> MELIKGQALFLELDKKDFLSLKNNDKNIPTFA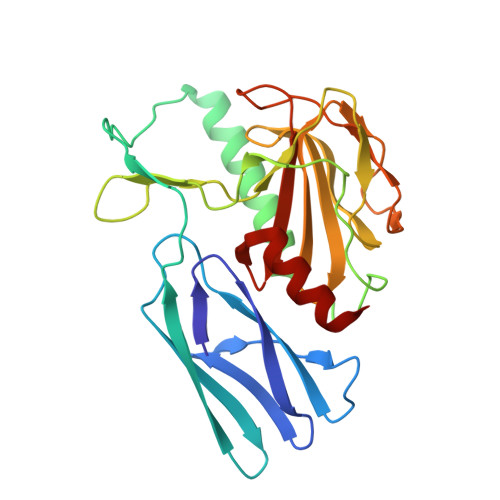HPKNQEKILAIFSLPYKNPPQNTKLIAFYKDKKEEIFIKTLEGNYKSEKLQVENKKIFPPKTIQERIAKELKEANAIYSSYTPKALFNGAFNIPLNSFITSDFGKARTFNEKVASYHSGTDFRAATGTPIYAANSGVVKIAKDRYFAGNSVVIDHGFGIYSQYYHLSKIDVKVGQKIKKGELIGLSGASGRVSGPALHFGILAGGKQVDPLDFVSKFNAIFQ>[2x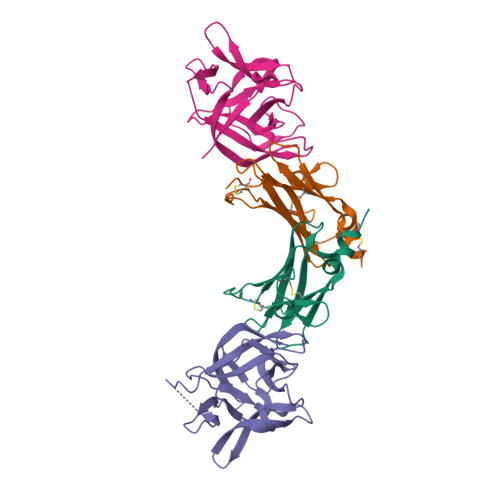]MECVKTRSVNIHVPVKETSKVVLECRGDSYFRHFSYVYWIIGKNKTVDQLPPNSGYRERIYLFKKPHRCENRPRADLILTNITDEMRNEKLTCVLIDPKDPLKESVILSKIWNCVYKI;>[2x]YFGKLESKLSVIRNLNDQVLFIDQGNRPLFEDMTDSDSRDNAPRTIFIISMYKDSQPRGMAVTISVASAAASTLSSENKIISFKEMNPPDNIKDTKSDIIFFQRSVPGHDNKMQFESSSYEGYFLASEKERDLFKLILKKEDELGDRSIMFTVQNED> MAALIDTGIFFGFYSLKDVHHMDSVAIVVHAVEGKWGRLFVTNHILDETLTLLKY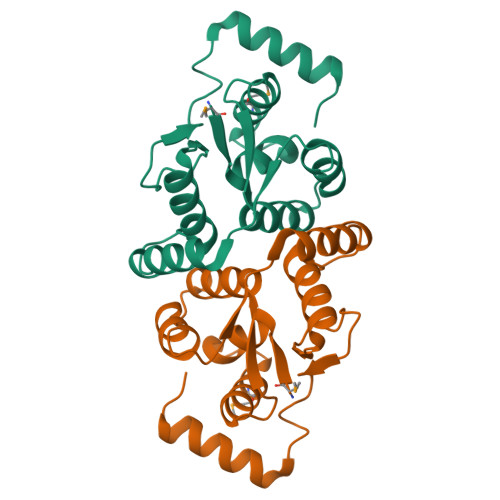KKLPADKFLEGFVESGVLNIIYTDDEVERKALEVFKARVYEKGFSYTDAISEVVAEELKLKLISYDSRFSLPTIGRDYWKSLDESERKRISAILREKGIDG(4-methoxyphenyl)(piperidin-4-yl)methanone 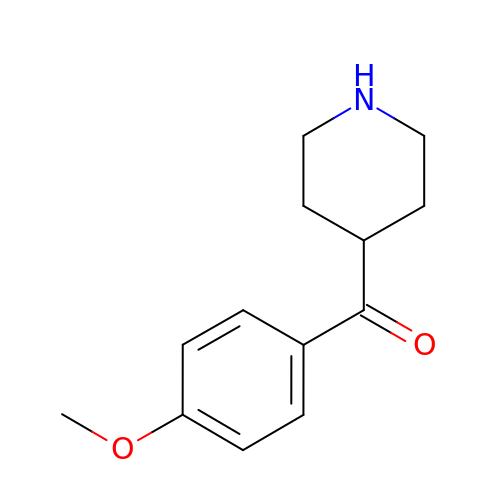| C13 H17 N O2 | ZYKYHSIACDLOCE-UHFFFAOYSA-N Using an X-ray free electron laser (XFEL), we have previously determined room-temperature (RT) serial femtosecond crystallography (SFX) structures of the ferric and Compound I redox states of DtpB,26 a B-type member of the dye-decolorizing peroxidase (DyP) family. Such an approach results in “pristine” DtpB structures that do not exhibit the effects of X-ray-generated radiation damage. The RT-SFX DtpB ferric and Compound I structures revealed that the distal heme pocket, which is composed of an Asp–Arg–Asn triad, was void of H2O molecules. DtpB, therefore, represents an exemplar of a His–heme-ligated peroxidase in which the distal heme pocket favors a dry site. By disrupting the distal heme pocket Asp–Asn–Arg triad in DtpB, our RT-SFX structures reveal that a wet site can be formed.

To assess whether disruption of the Asp–Arg–Asn triad in DtpB leads to a wet distal heme pocket, microcrystals of each variant in the Fe(III)–heme state were produced and subjected to RT-SFX crystallography using a high viscosity extruder sample delivery system at the SACLA XFEL beamline BL2 EH3. For all variants, well-defined electron density peaks were present in the distal heme pocket, consistent with the presence of resident H2O molecules. In the D152A variant, three resident H2O molecules are accommodated, with two occupying the space left by the Asp152 side chain. In the D152A, D152A/N245A, and R243 variants, w1 is positioned close enough to the heme–Fe(III) to be a bonding interaction (average Fe(III)–OH2 distances within the DtpB hexamer assembly of 2.52, 2.83, and 2.28 Å, respectively). An obvious feature is that WT DtpB displays a single pKa, as opposed to the D152A and double variants, which display two pKa values. In the D152A and double variants, H2O2 would be expected to replace w1, leaving two water molecules in the pocket, both of which participate in an extended H-bonded network, thus supporting a view that H2O dipole orientations can compensate for a proton remaining on Fe(III)–H2O2 and therefore increasing the pKa. Thus, the D152A and D152A/N245A variants (fully wet) are almost fully populated at 76 and 93%, respectively, while the “semi-dry” N245A variant is 52% populated. Therefore, we conclude that by disrupting the Asp–Asn dyad, a wet distal heme pocket forms in the Fe(III)–heme state, which does not influence the efficiency of DtpB reacting with H2O2, indicating that Arg243 facilitates Compound I formation in DtpB regardless of whether the pocket is wet or dry.

>[6x]MGGEVEEPEPQMVLSPLTSAAIFLVVTIDSGGEDTVRDLLSDVASLERAVGFRAQPDGRLSCVTGIGSEAWDRLFSGARPAGLHPFRELDGPVHRAVATPGDLLFHIRASRLDLCFALATEIMGRLRGAVTPQDEVHGFKYFDERDMLGFVAGTENPTGAAARRAVLVGAEDPAFAGGSYAVVQKYLHDIDAWEGLSVEAQERVIGRRKMTDVELSDDVKPADSHVALTSVTGPDGSDLEILRDNMPFGSVGREEFGTYFIGYARTPEVTETMLERMFLGTASAPHDRILDFSTAVTGSLFFTPAADFLEDLSARP(3S)-N-methyl-N-phenylpyrrolidine-3-carboxamide | C12 H16 N2 O | 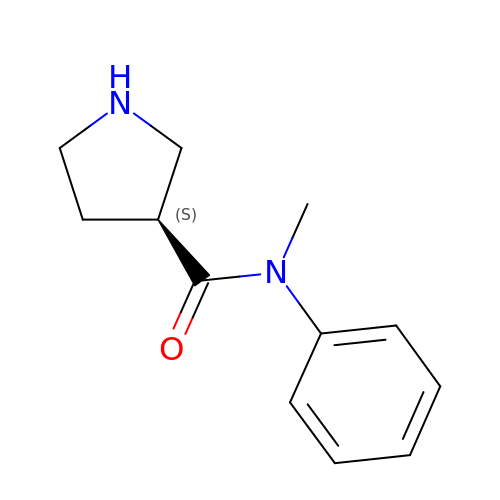VZIWWLIHHFDZEO-JTQLQIEISA-N> EDVRIQIWHQMIYGHRQVLAEALEKFEKENPGITVQATYRETEELRSSFQSAAMGGSGPELVYGPSDQVGPFATMGIVRPLDEVLGSDYFQNFDPLAAPVYDGKHYMIGDAVGNHLMLLYNKKFITTPPKNSQELIELGKKMTVDTNGDGKIDRWGLVFNYTEPFFFAPFIPAFGEAFLKADGVTPNLNTTALKDTFQFILKLRDQDKIIPKECDYETANALFKENKAAMLINGDWSWGDYQQAKVDFGIARIPMISETGKWPSPLVGTKGYSLNANMKSEAHYEAAVKLLKYLTSTPVQLLFAEKVGVLPSNLQARESDIVKNNPLLKISADIMEVGTPMPVTPEVRAVWDSLRIQYQKVLAGSLQPQAAAEQAQI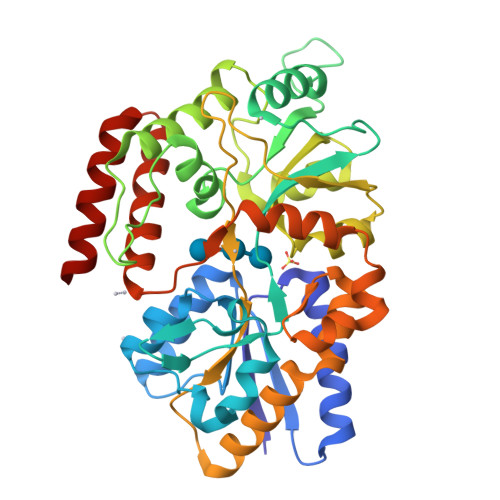TAEQQIRDMNE>[3x]GHMPLTQTQRLINTYGASLKNGTISNEELIILLDPNTFTKSEGYVDPNAPVSDSNHSKMDAIKDFVLTIGPTLDSEILHQLTSRMIELSPPGDRNTFMRGSSLEKAFLAFEMAH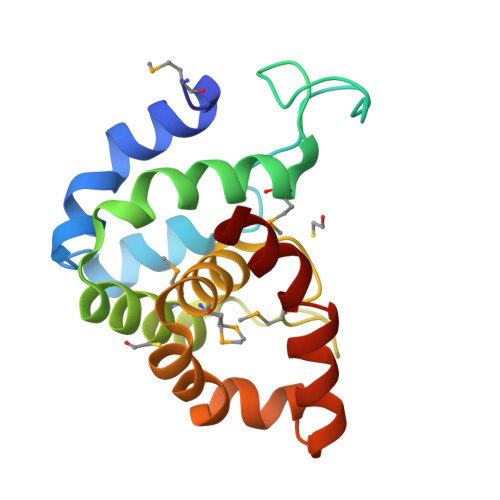YPTKAEEHFNSTRVRTEFPGENDIDNLKAVILNPIIAFFQS>SAIRSDFSNEDIYDNIDPDTISFPPKIATTDLFLPLFFHFGSTRQFMDKLHEVISGDYEPSQAEKLVQDLCDETGIRKNFSTSILTCLSGDLMVFPRYFLNMFKDNVNPPPNVPGIWTHDDDESLKSNDQEQIRKLVKKHGTGRMEMRKRFFEKDLL[2x];> SEKGNAKMIDFATL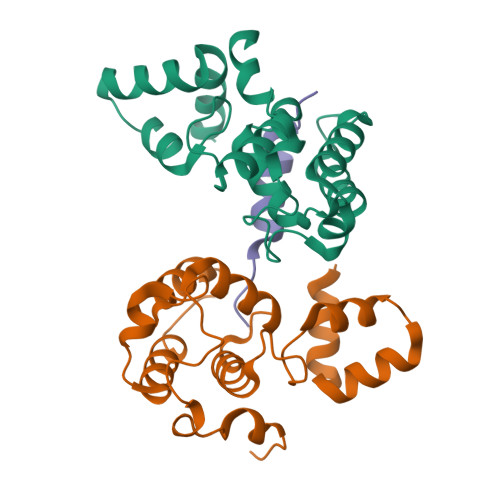SKLKKKYQIILDR>MEKMSSGTPTPSNVVLIGKKPVMNYVLAALTLLNQGVSEIVIKARGRAISKAVDTVEIVRNRFLPDKIEIKE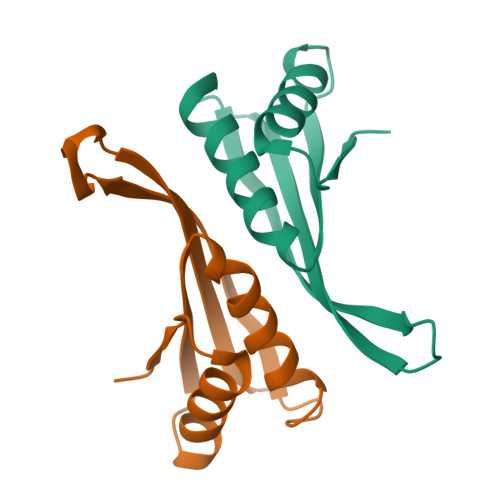IRVGSQVVTSQDGRQSRVSTIEIAIRKK[2x]> LRGS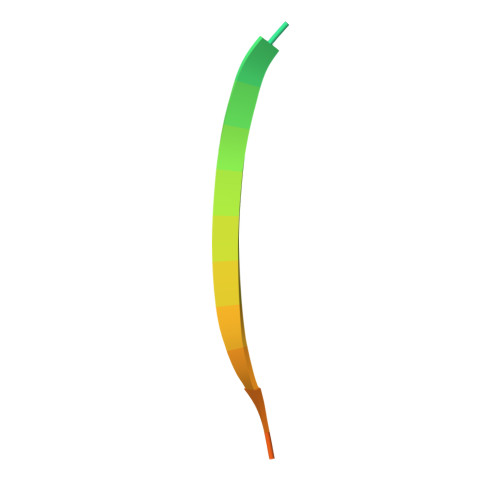LPTFRSSLFLWVRPNGRV> GSHMDNQCTVQVRLELGHRAQLRKKPTTEGFTHDWMVFVRGPEQCDIQHFVEKVVFWLHDSFPKPRRVCKEPPYKVEESGYAGFIMPIEVHFKNKEEPRKVCFTYDLFLNLEGNLNHLRCEKLTFNNPTTEFRYKLLRAGGVMVMPEGAH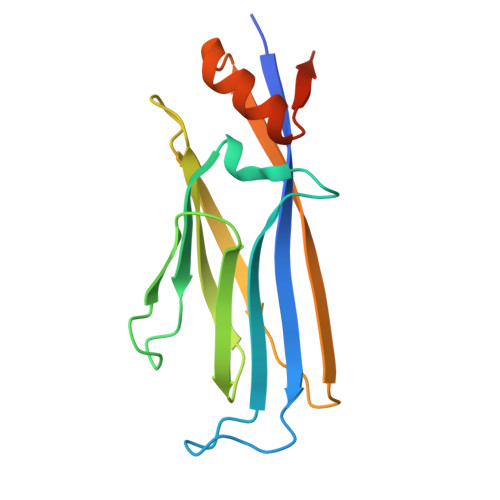HHHHH>[7x]MGSDKIHHHHHHM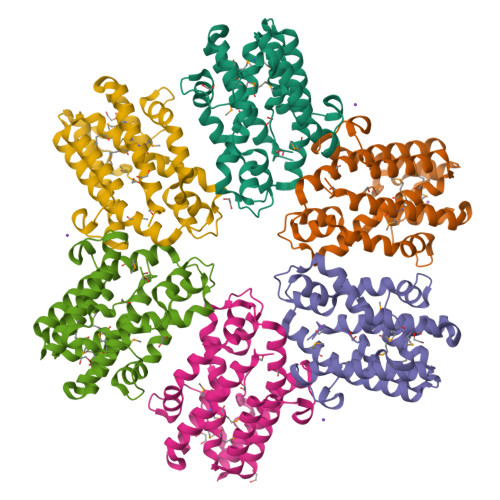NDFKNQWLRKRTFAIPASRLTGRLTTLKSDVPAADSLFWKLWNGSLDTAVQVLQTDYFKGIAAGTLDPNAYGSLMVQDGYYCFRGRDDYATAATCAQDETLREFFKAKAKSYDEYNETYHQTWHLREASGLIPGTDIKDYADYEAYVAGSLASPYMCVVMLPCEYLWPWIANFLDGYTPTNSLYRFWIEWNGGTPNGAYQMGNMLEQYRDKIDEDKAVEIFNTAMNYELKVFTSSTILTTIENGK>[2x]GDDEEADDPIRMYFEPGHYTVMENCGEFEVRVVRRGDISTYASVEYETQDGTASAGTDFVGRKGLLSFPPGVDEQRFRIEVIDDDVFEEDECFYIRLFNPSEGVKLAVPMIATVMIL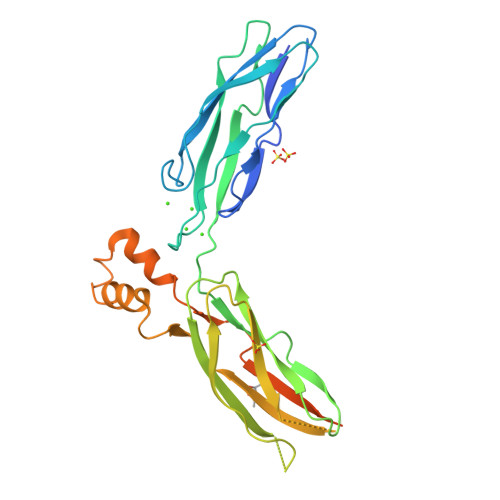DDDHAGIFAFTDSVFEITESVGRFELKVMRYSGARGTVIVPYWTENDTATESKDYEGARGELVFENNESEKFIDLFILEESSYEKDVSFKVHIGEPRLAPDDELAAKIKEVEKKPVQDLTELDRILLLSKPRNGELTTAYVRIRESQEFKATVDKLVAKANVSAVLGTSSWKEQFKDALTV> MARSPGRAYALLLLLICFNVGSGLHLQVLSTRNENKLLPKHPHLVRQKRAWITAPVALREGEDLSKKNPIAKIHSDLAEERGLKITYKYTGKGITEPPFGIFVFNKDTGELNVTSILDREETPFFLLTGYALDARGNNVEKPLELRIKVLDINDNEPVFTQDVFVGSVEELSAAHTLVMKINATDADEPNTLNSKISYRIVSLEPAYPPVFYLNKDTGEIYTTSVTLDREEHSSYTLTVEARDGNGEVTDKPVKQAQVQIRILDVNDNIPVVENKVLEGMVEENQVNVEVTRIKVFDADEIGSDNWLANFTFASGNEGGYFHIETDAQTNEGIVTLIKEVDYEEMKNLDFSVIVANKAAFHKSIRSKYKPTPIPIKVKVKNVKEGIHFKSSVISIYVSESMDRSSKGQIIGNFQAFDEDTGLPAHARYVKLEDRDNWISVDSVTSEIKLAKLPDFESRYVQNGTYTVKIVAISEDYPRKTITGTVLINVEDINDNCPTLIEPVQTICHDAEYVNVTAEDLDGHPNSGPFSFSVIDKPPGMAEKWKIARQESTSVLLQQSEKKLGRSEIQFLISDNQGFSCPEKQVLTLTVCECLHGSGCREAQHDSYVGLGPAAIALMILAFLLLLLVPLLLLMCHCGKGAKGFTPIPGTIEMLHPWNNEGAPPEDKVVPSFLPVDQGGSLVGRNGVGGMAKEATMKGSSSASIVKGQHEMSEMDGRWEEHRSLLSGRATQFTGATGAIMTTETTKTARATGASRDMAGAQAAAVALNEEFLRNYFTDKAASYTEEDENHTAKDCLLVYSQEETESLNASIGCCSFIEGELDDRFLDDLGLKFKTLAEVCLGQKIDINKEIEQRQKPATETSMNTASHSLCEQTMVNSENTYSSGSSFPVPKSLQEANAEKVTQEIVTERSVSSRQAQKVATPLPDPMASRNVIATETSYVTGSTMPPTTVILGPSQPQSLIVTERVYAPASTLVDQPYANEGTVVVTERV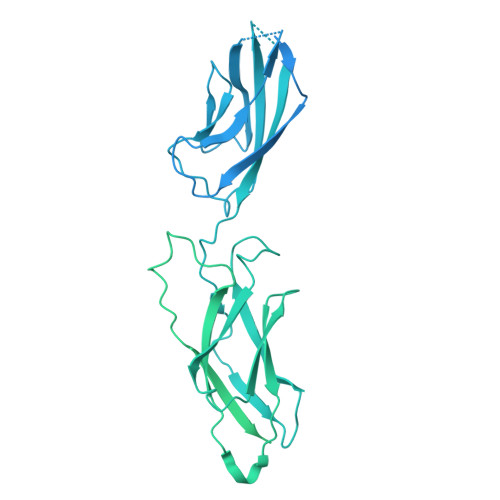IQPHGGGSNPLEGTQHLQDVPYVMVRERESFLAPSSGVQPTLAMPNIAVGQNVTVTERVLAPASTLQSSYQIPTENSMTARNTTVSGAGVPGPLPDFGLEESGHSNSTITTSSTRVTKHSTVQHSYS>[2x]MNENEPVSIWMHPEPAGRRSARSHRTLSRDQIVRAAVKV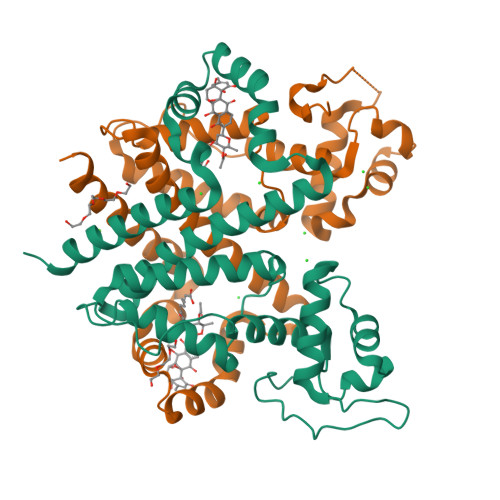ADTEGVEAASMRRVAAELGAGTMSLYYYVPTKEDLVELMVDEVIGETRLPDRPGPDWRAALTLAANEKRALWLRHPWLATAWRNGHPVWGPNSLRQQEFVLGTLGVFDLQVDELLSLIGLYNGYVESFVRNEVGWLEEARRTKVDMREWMRRSGPYAQQLVDSGEYPMFARVLAETVAPHMGPDQRFRSGLERLLDSIGASLDRLSPPGRSAASERPALALEHHHHHH>[7x]GSAKDVKFGADARALMLQGVDLLADAVAVTMGPKGRTVIIEQSWGSPKVTKDGVTVAKSIDLKDKYKNIGAKLVQDVANNTNEEAGDGTTTATVLARSIAKEGFEKISKGANPVEIRRGVMLAVDAVIAELKKQSKPVTTPEEIAQVATISANGDKEIGNIISDAMKKVGRKGVITVKDGKTLNDELEIIEGMKFDRGYISPYFINTSKGQKCEFQDAYVLLSEKKISSIQSIVPALEIANAHRKPLVII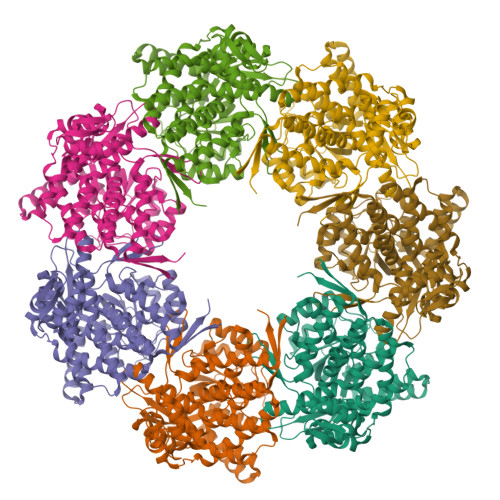AEDVDGEALSTLVLNRLKVGLQVVAVKAPGFGDNRKNQLKDMAIATGGAVFGEEGLTLNLEDVQPHDLGKVGEVIVTKDDAMLLKGKGDKAQIEKRIQEIIEQLDVTTSEYEKEKLNERLAKLSDGVAVLKVGGTSDVEVNEKKDRVTDALNATRAAVEEGIVLGGGCALLRCIPALDSLTPANEDQKIGIEIIKRTLKIPAMTIAKNAGVEGSLIVEKIMQSSSEVGYDAMAGDFVNMVEKGIIDPTKVVRTALLDAAGVASLLTTAEVVVTEIPKEEKDPGMGAMGGMGGGMGGGMF> PLVWTQLKQTGTTQPTARSGHTIITVGKTHIMFGGLDNDKNNYKDGKIAPNNQVFTLKLTQNNCEWRQIACQGDVPLPRCYHASCAISADKMLVFGGSYTSNLRFNDTYILKTTSYQWSKPANQISGGEPKNAESKIGAPQPRYGHSATFFEGKVYIFGGHGGINYQRLAFNDLYVLETENFEWTRLEPKGNPPDPRGGHSAAMMANKPQLMIFGGWSFTSQYSNIMIYDIEKDEWVDPEIAHEIPKWNLSGIMAPSIPSWKYFIFGGSVGSFEEGGNRTNSRFVDDSFVLDIDTLSWSSINLEADETSKAVCKPRPRESASIFYDSGESRAIVFGGWANNWLNDLWALNVSTITGPIFSIKPALGPLTGKTKVLIEGDGFKDTQNISVKFSGGKLEKEVNGTFVNEKEISCETPTFDYPRSVEVTVCMNKGDYTITKSAFTYTKADKTIAYGPGLLTENLIGVQTTIVIQARNGSDEFVVTIRNPAKIKKEEEVKEGDKANTKNTIKEDEEEEGEDEEENKKKKEAEKNDLTGSAVMNYISKQLKDIQEFIENTKENIEIRNKNISELINVMINLEKVRVKNDDDVLTLDTVEEMLNFLKKKKDSDIKKCKKLQEEWKNLAKMAQAVKKDIQNPVKTESDKTKENIKKFEEITLKEYANSLKKESFYKTGVSESFKRIGEVKQKVDEFEVQLNQYEDFARIGSKKLMEQIRTDVSSVEKLWVRIEISEKTMDEYKKM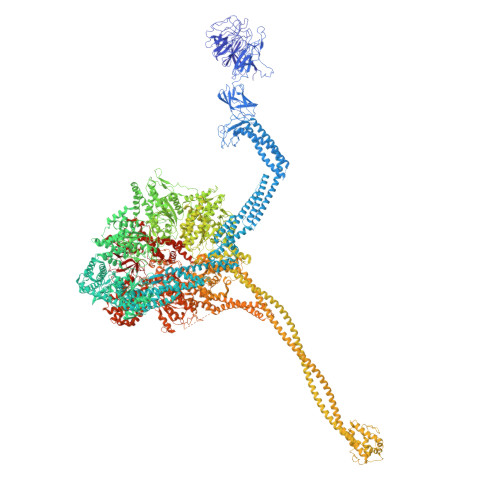KWGSINSMDMEDEIKKLRKALTDLRGIDKRSNAFIGITEELKKWATFLPLLGELKDPSMNSEDGRHWKKLKDLVKKEFDVSQELMLEIIWDLKLFDYKDGIEEITDQAKQELKMEKALKKIIDFWRDIEFELVQHKNTDIHTLKMSEENFETLEDHQLQINNMLLSKYVAYFEKEVEKWKYDLGSVYDVVQLLLEVQKTWSFLENLFEVKRELPNESAQFVGIDKDMKEIMQKGCDIKNCLKFCTIEGMLKRLENIQAQLKVCEKALNEFLDSKRRAFPRFYFVSVNDLLDILSNGNSPAKINRHMSKIFQAIDNLQLKEDSSGGRPTLKMISCVGTEEVDFSSPRLLQGKVESYLKDVIDTMIGTLKSVANSSFKNFQSMTRKEWLKSDPSQITLLVNNIIWSKAVEDCFLKLQSGDINAMKLFLDESIKQLTELIGMVQGDLSKPLRQKIMCLITIDTHSRDVVHRLINEHVRKAEEFQWQSQLKFYWVDNDAKIKIADARFVYNYEYLGNGPRLVITPLTDRIYVTATQALHLKMGCAPAGPAGTGKTETTKDLANALAKACYVFNCSSEMNYESMGNIYKGLASSGCWGCFDEFNRLLPEVLSVCSVQFKAVTDAIKQNVERFIIEGDEISLDPTCGVFITMNPGYLGRAELPEGLKALFRPITVVVPDLELICENMLMAEGFIEAKILAKKFVTLYMLCRDLLSKQLHYDWGLRAIKSVLVVAGGFKRSEPEIAEQALLMRALRDFNIPKIAFQDLYVFHGLLGDLFPGINIKPKKDLDFEKIITDVCIENKLDPDPEFVLKVVQLSELLAIRHCVFVMGPPGAGKSTTWKILAKAQDKTNKKTTLIDIDPKVVSTKDFYGYNLPSKEWKDGLFSKMLRSLAEQPDTNPKWICLDGDLDANWIESMNSVMDDNKILTLANNERIPLKPHMRALFEIRDLRFATPATVSRAGILYISDEVGYQWRSYVKSWIKQEFSQDQEMSKNLDTLFGKYVPDTLDHIKKHCRFLVPVSPISQVISICKSLQTLLKGDVKNLEYLFVYALIWAIGGALAEKDSIDYRKDFSTWWKGAWKTAVKFPSKGTIFDYYVDQSGDSSKFVEWSKRLENKEFDPQVETMGNITVNTIETLATTEFIKSYLMVKHPSLLIGNSGCGKTQLAKGILKEIVQAKPENYAYQLINFNYYTDSTYLQGQIEQTLEKKAGRQYGPPGKVQLIYFIDDLNMPQLDAYDTQTAIALLRQLADYGHFYDVSKLALKDIINTQVLAAMNPSAGSFFVNPRYQRHFWTISIPFPDNESLSLIYITFLNGHLKRFKSTIQEYSNIIVRASLMLHQAVTQNFRKTAINFHYEFNLRHMSNVFQGLLLSDPNKFTEPDKLIKLWIHECERTYGDRLVSTDNLKTYKENIFDIVKKSFSKFNFSRYFGNNPENLIYCNFIAGINSDRFYDQMPNNEMEKHISEALKEYNDNNAFMGLVLFEDAMKHVCRICRIVLPSSGHALLVGVGGSGKQSLSKLASFIMGYTTFSITISATYSMVDLRNDLQQLYFKCGPKEEGILFLFTEGQITNERFLVYINDLLSSGEIAELYTLDEKEAMINQVRAKVKGEGKPDTRENCWNWFIDQVKKNLHMAICFSPVGDMRRRARQFPALVNCTVIDWFQPWPYEALFNVAKSFLEPVDLGDDKVREAVVKFMPFSFTLVNDLGLKLLEQERRYAYTTPKSFLELISLFTNMLAQKRESLERNKERYETGLVKLKETAEQVAIIEVEVKEKQVEAEAKKKEADAFAEVVGREKDKVEKENSKATIEADKCGLIKQNVEAQKSSTQQDLDAAQPLVEQAKSALNSISKKDFQQAKSFASPPAGVPEVFAATIYLLAGYFNEAIEIDKNKKPKDVSWKSSLKLMKSPEEFMEKLLNFKDVVDANQVANVNIVKNQYLNMPSFTPEQMASKSAAAKGICSWVVNIVKYYDVIQDVEPKRKALKEATEQLEEATVKLNEVEEVVRKLNEELNKLKAENDKAIAERNAAISEAERCARRLNLAQRLVTALSSENERWGKSIIQLEDQLKLMVGDVLVASSFVSYSGPFNKKFRNIMINQNFMKFMKEHTIPMSPDPNPIKILTDESTIALWNKQKLPSDSVSIENGTILTNSARYPLMIDPQLQGITWIREKEKANNLKILRLGSKNINRDLELSIENGYSAIIENMNERIDAILMPIIARSFIKRGKNKIIKFAGKDLILHPNFKLFLHTKLSNPHYPPEIQAEAALINFTVTEAGLGDQLLSLVVARERPDLAKMKIELITQQNDFKIKLKDLEDELLYKLANAKGDILDDIELIENLEYSKKLSVEIAEKVAAAKITEAKINETSENYRPAASRGALFYFLLSDLSKVHSFYKYSLESFIVVINRAIDAISENKIYGKTTMMSPRSLKKRVDELIESLTYTAYQTTRRGLFESHKLIVAAMLCLRVLLRSEELNSDEVDHLIIGKVDVNPTPMPDALKSFLNDNIWAACKALETIHQFQGFCQSLETDVLQWKKWYSEEKAETADLPKAFKELSKFHRLLLLRALRPDRLPSALSQFVHDKMGERYIEQPPFNIFETFQETSKTVPIFFVLFPGVDPTPDVERVAATFDVSANNGRFINISMGQGQEDRAKKALFDCAQKGHWIMLQNVHLMQSWLYGLNGLEGFLESVFASPKTHPNFRVFISSEPPNVLLPLMQIIPESILQGSLKIANEAPQYLKANLRRAYNKFDQEFLDKCDKKPTEFKSCLFALCFFHSLMLGRKKFGTQGWSRVYNFNDGDLTICADVLYNYLSKYDQVPWDDLRYIFGEIMYGGHITDDWDRRTNRTYLKVLIRSELLQQNFNLAPQFKSPDPSKFDYEAYRKYIEEKLPIESPQMFGMHPNAEIGYLTQTCDQVFNTILEVQGGSSGGGASKKDDGVMVTLTDFKTRCPHDFNMLLIEEKVKEKTPYIVVCLQECERMNGLLKEIKTSLEDLRLGLTGALNMTDAMESLQQSLSFNKVPDTWEKKAYFSKKPLSSWFADLIERNIQLQEWCKELVTPTSLCISYLFNPMSYLTAIMQFTARAQGLPLDGITIQTNVTAMKGPEDVVNPAENGAYIHGLFLEGAAWEIGGQGQDGYLIEQKPKELHPKMPVINAVAVPLDKKKKNGQYDCPTYVTSARGQTFVFTANLNMESDDSDPNKWILSGTCMLMSDD> KKATATTWMVPT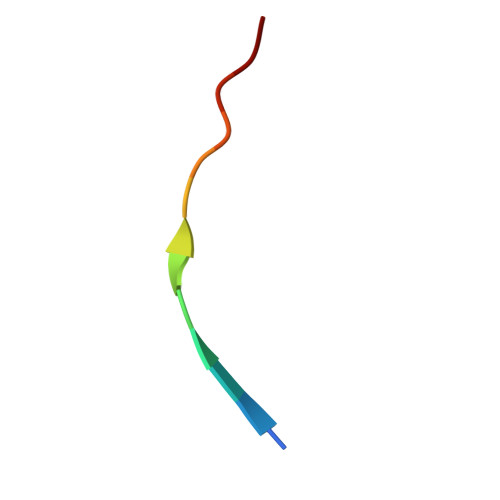A During HR, a recombinase binds to single-stranded DNA (ssDNA) and forms a right-handed helical nucleoprotein filament, known as a presynaptic filament, which then searches double-stranded DNA (dsDNA) for homology. Eukaryotic RAD51 and DMC1 both catalyze strand displacement and strand exchange. Interestingly, DMC1 possesses the ability of stabilizing mismatch-containing recombination intermediates (low-fidelity recombinase), whereas the RAD51 lacks the ability to do so (high-fidelity recombinase). RAD51 and DMC1 are members of the RecA family of DNA recombinases and share ~50% amino acid identity and similar biochemical properties.

We first solved the cryo-EM structures of human DMC1 filaments with ssDNA and dsDNA (homologous) in presynaptic and postsynaptic states (Structure 1, 3.33 Å and Structure 2, 3.47 Å, respectively), in the presence of adenylyl-imidodiphosphate (AMP-PNP) and Ca2+. Similar to the corresponding complexes of RAD51, both structures adopt a well-ordered helical structure, with six protein protomers interacting with six triplets of DNA. The bound DNA is organized into near B-form base triplets separated by ~8 Å between adjacent triplets.

>[3x]MKEDQVVAEEPGFQDEEESLFQDIDLLQKHGINVADIKKLKSVGICTIKGIQMTTRRALCNVKGLSEAKVDKIKEAANKLIEPGFLTAFEYSEKRKMVFHITTGSQEFDKLLGGGIESMAITEAFGEFRTGKTQLSHTLCVTAQLPGAGGYPGGKIIFIDTENTFRPDRLRDIADRFNVDHDAVLDNVLYARAYTSEHQMELLDYVAAKFHEEAGIFKLLIIDSIMALFRVDFSGRGELAERQQKLAQMLSRLQKISEEYNVAVFVTNQMTADPGATMTFQADPKKPIGGHILAHASTTRISLRKGRGELRIAKIYDSPEMPENEATFAITAGGIGDAKE>EEVRQFRRLFAQLAGDDMEVSATELMNILNKVVTRHPDLKTDGFGIDTCRSMVAVMDSDTTGKLGFEEFKYLWNNIKKWQAIYKQFDVDRSGTIGSSELPGAFEAAGFHLNEHLYSMIIRRYSDEGGNMDFDNFISCLVRLDAMFRAFKSLDKDGTGQIQVNIQEWLQLTMYS[2x];>[2x]DAIDALSSDFTS;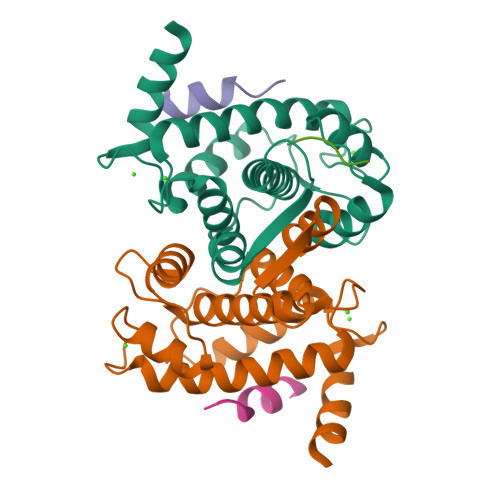> AKAIA6-(3-TETRADECANOIC ACID) FLAVINE MONONUCLEOTIDE | C31 H47 N4 O11 P | 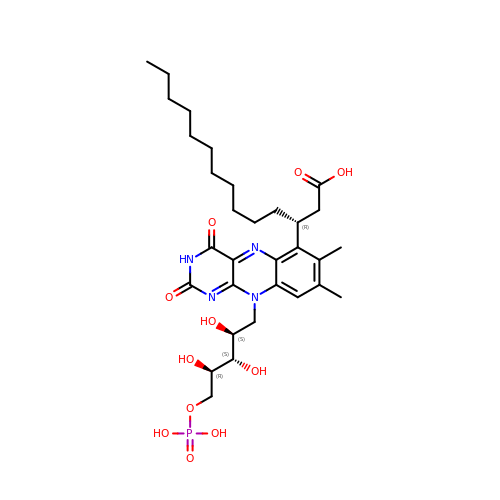ZMESPPGIOMLBCU-QPLRPWAESA-N>[5x]MKSLLRQIPQISKVVEIFAKAYPEIYVVKAAREVAEKYRKEIIEGARADLNGFLEDVERKIKSLMKPN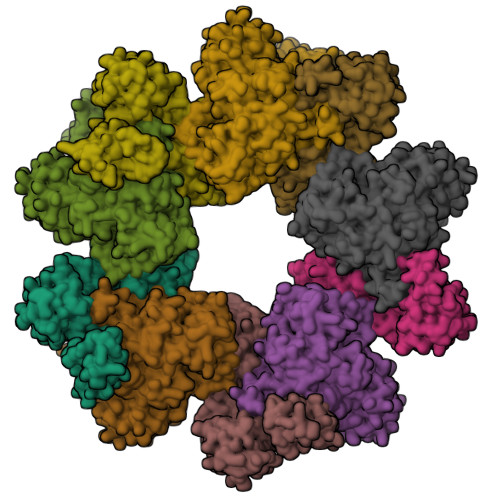IKRVINATGVVINTNLGRAPLSKDVINFISEIANGYSNLEYNLEEGKRGSRIAHIEKYLNELTGAESSFVVNNNAGAVFLVLNTLAEGKEVIISRGELVEIGGSFRIPDIMKKSGAILREVGTTNKTKVSDYEGAINQNTALLMKVHKSNFYMEGFVEEVKLEDLVKLGHKYGIPTYYDAGSGLLINLKEFGISVDEPNFRDCISLGIDLVSGSGDKLLGGPQAGIIVGKKNLIEKIKKNPIARALRIDKLTLSGLEMTLKLYFEKRYEDIPVIRMLTQDEKALRQKAKRLEKLLKDIPGLKISVIKDKAKPGGGSLPELELPTYCVAIRHDRLSSQELSRRLRLAEPPIVCRIREDQLLFDMRTVFHEDLKTIKKTLQELLSI>MRVLLIAGGVSPEHEVSLLSAEGVLRHIPFPTDLAVIAQDGRWLLGEKALTALEAKAAPEGEHPFPPPLSWERYDVVFPLLHGRFGEDGTVQGFLELLGKPYVGAGVAASALCMDKDLSKRVLAQAGVPVVPWVAVRKGEPPVVPFDPPFFVKPANTGSSVGISRVERFQDLEAALALAFRYDEKAVVEKALSPVRELEVGVLGNVFGEASPVGEVRYEAPFYDYETKYTPGRAE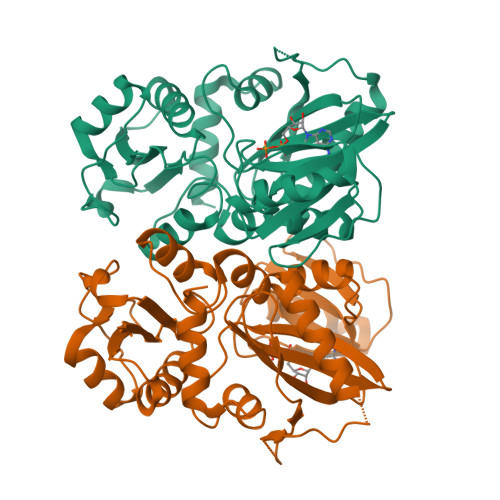LLIPAPLDPGTQETVQELALKAYKVLGVRGMARVDFFLAEGELYLNELNTIPGFTPTSMYPRLFEAGGVAYPELLRRLVELALT[4x]> TQKSLSKEEIERYSRQMIVPGMGKEGQLRLMNAKVLIIGAGGLGCPAAQYLAGAGVGTIGIVDGDSVETSNLHRQVAHATKRVGMLKVDSLITHLIEINPLPVYVPYRFDLTPQNAAQIIKPWDVILDCTDNPATRYLISDVCVLLGKPLVSAASVQKSGQLIVLNCPPTPQGVVNKKAAPCYRCCFKKPPPPSAQTSKGEAGIMGPVVGMMGVAQAGEAIKILVSQLHMPPKEGEEVSPEKNLVQPTLLIYTYDLNSAIGPYSFRALKMGGRKKDCFACGENSTLTLDGIKSGNPNYVQF;> IPITVDFSGGLEMLFDNQRRHSISLPAKDTEGKPVTIAFLIDYICKKLMKDP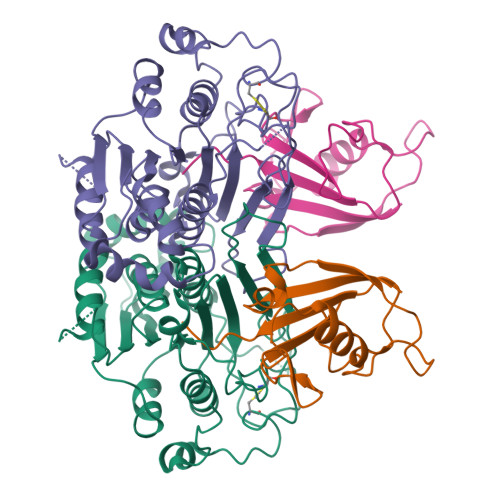RTDLFVLDNHIRPGILVLINDADWELEGEEAYEIQPNDNILFVSTLHGG>DSVYVQNPQIPILVDRTDNVLFRIRIPDATKGDVLNRLTIRFGNEDKLSEVKAVRLFYAGTEAATKGRSRFAPVTYVSSHNIRNTRSANPSYSIRQDEVTTVANTLTLKTRQPMVKGINYFWVSVEMDRNTSLLSKLTSTVTEVVINDKPAVIAGEQAAVRRMGIGVRHAGDDGSASFRIPGLVTTNKGTLLGVYDVRYNNSVDLQEHIDVGLSRSTDKGQTWEPMRIAMSFGETDGLPSGQNGVGDPSILVDERTNTVWVVAAWTHGMGNARAWTNSMPGMTPDETAQLMMVKSTDDGRTWSESTNITSQVKDPSWCFLLQGPGRGITMRDGTLVFPIQFIDSLRVPHAGIMYSKDRGETWHIHQPARTNTTEAQVAEVEPGVLMLNMRDNRGGSRAVSITRDLGKSWTEHSSNRSALPESICMASLISVKAKDNIIGKDLLLFSNPNTTEGRHHITIKASLDGGVTWLPAHQVLLDEEDGWGYSCLSMIDRETVGIFYESSVAHMTFQAVKIKDLIR[2x]

The NanH sialidase of Tannerella forsythia, one of the bacteria associated with severe periodontal disease plays a role in virulence. The C-terminal catalytic domain is preceded by a 160 amino acid N-terminal domain that is a CBM that our laboratory discovered is capable of binding various sialoglycans and non-sialylated derivatives but has no catalytic activity itself. The NanH catalytic domain (residues 197–552) folds into a characteristic 6-bladed β-propeller catalytic domain, with each blade being composed of 3–4 antiparallel β-strands.

Using our established protocol for producing highly purified and concentrated enzyme, NanH was screened in sitting-drop crystallisation trials, with conditions containing protein in 0.1 M HEPES pH 6.0, 7% w/v PEG 6000 producing robust crystals. The model consisted of 519 residues (34–552) in each subunit and showed that there were two copies of NanH in the asymmetric unit. The location of the active site in NanH is highlighted by the presence of the conserved catalytic residues at the centre of the propeller, where D237 is the conserved aspartate, which is believed to be involved in the catalytic mechanism along with Y518 and E407, which are likely the nucleophile and acid–base residues, based on structural homology. Surprisingly, in our first crystal form, the active site was occupied by a molecule of HEPES (shown in yellow), with its sulfate group occupying the predicted position of the sialic acid carboxyl group expected from its location in other structures and being co-ordinated by R212, R423 and R487 that form an arginine triad. A lower concentration of HEPES in the crystallisation buffer of 0.01 M did result in subsequent datasets and maps to which a model was fitted that lacked the HEPES molecule but otherwise had identical features, implying that binding of HEPES did not cause changes in conformation. It is also notable that the NanH model shows a non-proline cis-peptide between residue L238 and Q239. In this region of the model adjacent to the cis-peptide in space, we also see an uncommon arginine rotamer (observed in other protein structures with ≤1% frequency) for R306. The data here reveal that the CBM is composed of 4 antiparallel β-strands that form the base of an open cleft.>[13x]CGKSEAPPPAQTPEVGIVTLEAQTVTLNTELPGRTNAFRIAEVRPQVNGIILKRLFKEGSD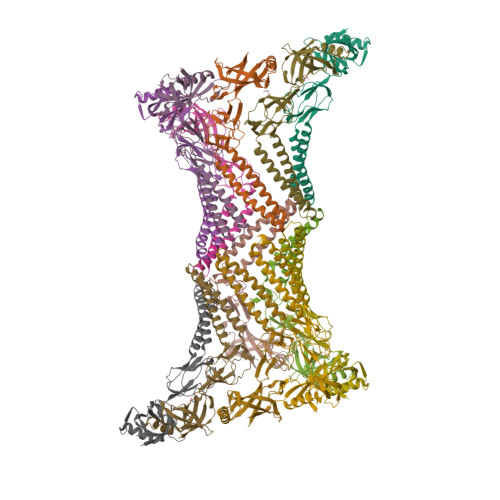VKAGQQLYQIDPATYEADYQSAQANLASTQEQAQRYKLLVADQAVSKQQYADANAAYLQSKAAVEQARINLRYTKVLSPISGRIGRSAVTEGALVTNGQANAMATVQQLDPIYVDVTQPSTALLRLRRELASGQLERAGDNAAKVSLKLEDGSQYPLEGRLEFSEVSVDEGTGSVTIRAVFPNPNNELLPGMFVHAQLQEGVKQKAILAPQQGVTRDLKGQATALVVNAQNKVELRVIKADRVIGDKWLVTEGLNAGDKIITEGLQFVQPGVEVKTVPAKNVASAQKADAAPAKTDSKG Here, the detailed functional and structural characterization of Thermus parvatiensis prophage peptidoglycan lytic amidase AmiP, a globular Amidase_3 type lytic enzyme adapted to high temperatures is presented. Endolysins can be divided into three groups (i) peptidases that cleave the amide bonds between amino acids; (ii) glycosidases capable of hydrolysing glycosidic linkage; and (iii) amidases cleaving the amide bond between N‐acetylmuramic acid and L‐alanine at the N‐terminal portion of the stem peptide in peptidoglycan mesh (Vermassen et al., 2019). The here presented AmiP constitutes the most thermoactive and ultrathermostable Amidase_3 type lytic enzyme biochemically characterized with a temperature optimum at 85°C. The extraordinary high melting temperature T m 102.6°C confirms fold stability up to approximately 100°C. Furthermore, AmiP is shown to be more active over the alkaline pH range with pH optimum at pH 8.5 and tolerates NaCl up to 300 mM with the activity optimum at 25 mM NaCl. The functional characterization of AmiP demonstrates high efficiency of catalytic activity and broad substrate specificity toward thermophilic and mesophilic bacteria strains containing Orn‐type or DAP‐type peptidoglycan.

Diffraction data were collected to a resolution of 1.79 Å and the structure was refined to a final R work 0.185 and R free 0.225. The structure solution by single‐wavelength anomalous diffraction revealed five independent AmiP molecules in the crystallographic asymmetric unit. The domain consists of a mixed α/β fold with a central six‐stranded β‐sheet surrounded by four α‐helices and nine loops. Helices α1, α3 and C‐terminal helix α4 shield the rear side of the β‐sheet, while helix α2 partly covers the β‐sheet front side. The active site is located in the shallow cavity of the upper end of an extensive recessed cleft defined by loops l1, l5, l8, and helix α2 across the β‐sheet. The Zn2+ ion in the catalytic site is coordinated by His17Nε2 (AmiP (B) 2.18 Å), His85Nδ1 (AmiP (B) 2.15 Å) and Glu32Oε2 (AmiP (B) 2.06 Å). One glycerol molecule (GOL) originating from the crystallization conditions serves as a bidentate ligand completing the Zn2+ ion distorted trigonal bipyramidal coordination geometry. Glu145 acting as catalytic residue located in strand β6 is oriented in proximity to the coordinated Zn2+ ion. Compared to these structures AmiP adopts a distinct compact organization achieved by omission of a helix α4′ and shortening of helix α3 as well as all β‐strands and loop l5. AmiP's compactness confirms a trait associated with adaptation to high temperatures as it was shown before that hyperthermophilic proteins are usually shorter than mesophilic homologues (Walden et al., 2004).

>MVRRQAPSAYIVLDPGHGGQDPGAVAPDGTREADLNLAQALTLKEYLVALGYRVGFTRTSDVYVPLSERIAMARRMGARLFISVHHDTPTASRPGVYYSPHPGSEELARTVAAALGEGAWVRPSSASRFGRLYIDDFPGPAILVEFGPTRPISRAERIARAQAVASPIAEFARRWTA[5x]>[6x]GAMRGSRKEPDKLKKVLDKLRLKRKDISEAAETVNKVVERLLRRMQKRESEFKGVEQLNTGSYYEHVKISAPNEFDVMFKLEVPRIELQEYYETGAFYLVKFKRIPRGNPLSHFLEGEVLSATKMLSKF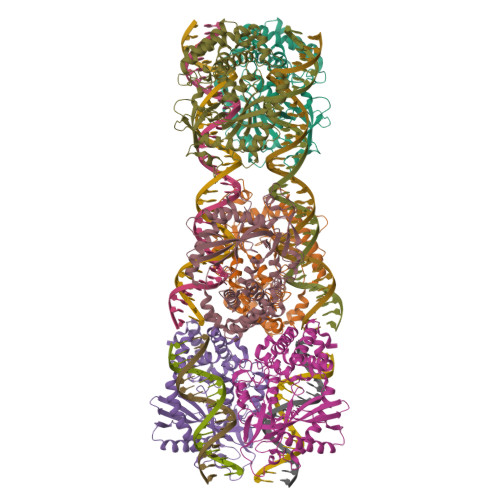RKIIKEEVKEIKDIDVSVEKEKPGSPAVTLLIRNPEEISVDIILALESKGSWPISTKEGLPIQGWLGTKVRTNLRREPFYLVPKNAKDGNSFQGETWRLSFSHTEKYILNNHGIEKTCCESSGAKCCRKECLKLMKYLLEQLKKEFQELDAFCSYHVKTAIFHMWTQDPQDSQWDPRNLSSCFDKLLAFFLECLRTEKLDHYFIPKFNLFSQELIDRKSKEFLSKKIEYERNNGFPIFDKL> AK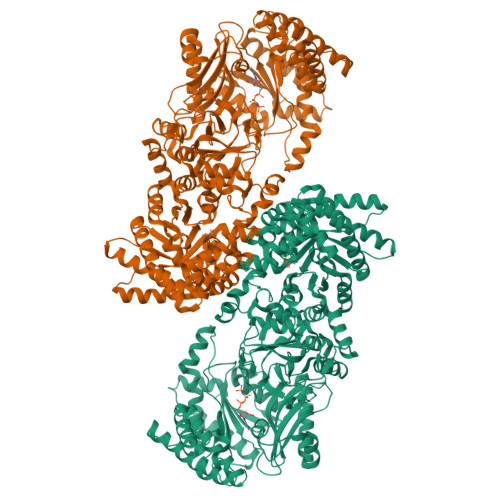KRVFTFGKGRSEGNKDMKSLLGGKGANLAEMASIGLSVPPGLTISTEACEEYQQNGKKLPPGLWDEILEGLRYVQKEMSASLGDPSKPLLLSVRSGAAISMPGMMDTVLNLGLNDEVVAGLAGKSGARFAYDSYRRFLDMFGNVVMGIPHSLFDEKLEEMKAEKGVHLDTDLTAADLKDLVEQYKNVYVEAKGEKFPTDPKKQLELAVNAVFDSWDSPRANKYRSINQITGLKGTAVNIQCMVFGNMGNTSGTGVLFTRNPSTGEKKLYGEFLVNAQGEDVVAGIRTPEDLATMETCMPEAYRELVENCKILERHYKDMMDIEFTVQENRLWMLQCRTGKRTGKGAVRIAVDMVNEGLIDTRTAIKRVETQHLDQLLHPQFENPSAYKSHVVATGLPASPGAAVGQVVFSAEDAETWHAQGKSAILVRTETSPEDVGGMHAAAGILTARGGMTSHAAVVARGWGKCCVSGCADIRVNDDMKVLTIGDRVIKEGDWLSLNGSTGEVILGKQLLAPPAMSNDLETFMSWADQVRRLKVMANADTPNDALTARNNGAQGIGLCRTEHMFFASDERIKAVRKMIMAVTPEQRKAALDLLLPYQRSDFEGIFRAMDGLPVTIRLLDPPLHEFLPEGDLEHIVNELAVDTGMSEDEIYSKIEKLSEVNPMLGFRGCRLGISYPELTEMQVRAIFQAAVSMNNQGVTVIPEIMVPLVGTPQELRHQIGVIRGVAANVFAEMGLTMDYKVGTMIEIPRAALIAEEIAKEAEFFSFGTNDLTQMTFGYSRDDVGKFLQIYLSQGILQHDPFEVLDQKGVGQLIKMATEKGRAANPNLKVGICGEHGGEPSSVAFFDGVGLDYVSCSPFRVPIARLAAAQVVV> MGIPAAFRWLSNKYPKIISPVVEERPIVMPDGTEIPVDATRPNPNGEEFDNLYLDMNGIVHPCSHPEDKPAPKDEEEMMIEIFKYTDRIVKMVRPRKILMIAVDGVAPRAKMNQQRSRRFRAAQEAKEKEEEKKQLLKMLRKEKGSNMQEEPLETVVKKAFDSNSITPGTPFMDILAASLRYWCAYKLNTDPAWAKLKVIISDATVPGEGEHKIMEFIRSQRSSPEHNPNTRHVIYGLDADLIMLGLATHEPHFRVLREDVFFQEAKARLCKLCGQKGHDERSCKGEAKQKQGEFDEKDHAQPLKPFIWLHVSILREYLAAELEVPNLPFRWDLERAIDDWVFLCFFVGNDFLPHLPALEIRENGIDTLTAIWKDNLPIMGGYLTKDGHVDLERAQYILNGLAKQEDAIFRRRREVEERREANAKRRKLNQQGAHAKGAADSHAGKSGR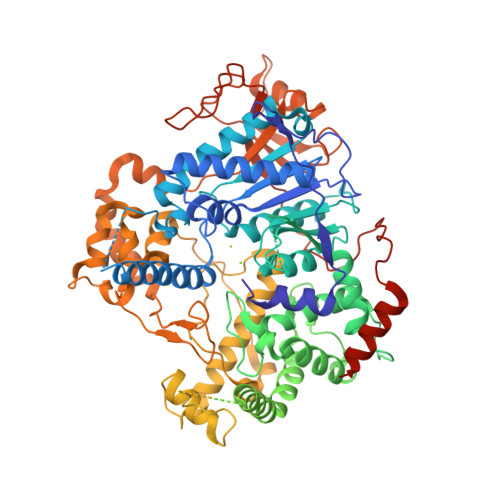KHVPEAAGPLPGMALFPITNPPPPAITHDMVMKGRSVDQANLANKSAASVLKSQIQSMMAQKAATNANGAEKDVSADGTTTAPASALGKRKAELIEEDAATNTDTDSVTDGTGSDNEGPVDTVRLWEEGYADRYYEQKFKVDPKDIEFRHKVGRAYAEGLAWVLQYYYQGCPSWEWFYPYHYAPFAADFVDLAKMEIKFEKGRISRPFEQLMSVLPAASRHAIPEVYHDLMTDPNSPIIDFYPEEFEIDLNGKKMAWQGVALLPFIEMPRLLAAMKEREHLLSEEDRARNEPGFDVLLISDAHPGLYEDITSHFYSKKQGAPKFKLNPRRSDGLAGKVEKIEGYVPHGSLVYPLARNSMPDVDYDRSITVRYIMPSSAHQHKSMLLRGVKLPPPALSRSDIEIIRSKAKNAGRSYGGAPLRNNYNSLEHHHHHH> MSLGTIIIVDDNKGVLTAVQLLLKNHFSKVITLSSPVSLSTVLREENPEVVLLDMNFTSGINNGNEGLFWLHEIKRQYRDLPVVLFTAYADIDLAV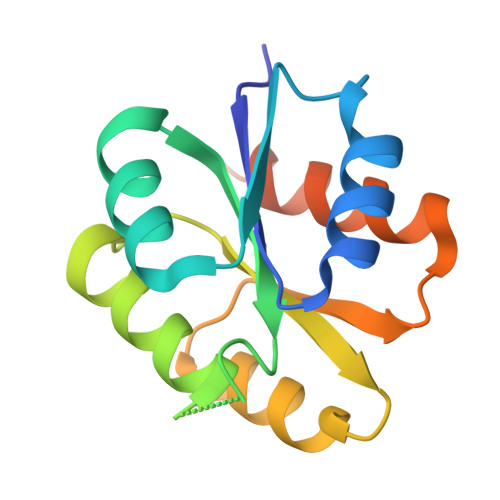RGIKEGASDFVVKPWDNQKLLETLLNAASQAKDGKKEGHHHHHH>GSHDYLFKLLLIGDSGVGKTCVLFRFSEDAFNSTFISTIGIDFKIRTIELDGKRIKLQIWDTAGQERFRTITTAYYR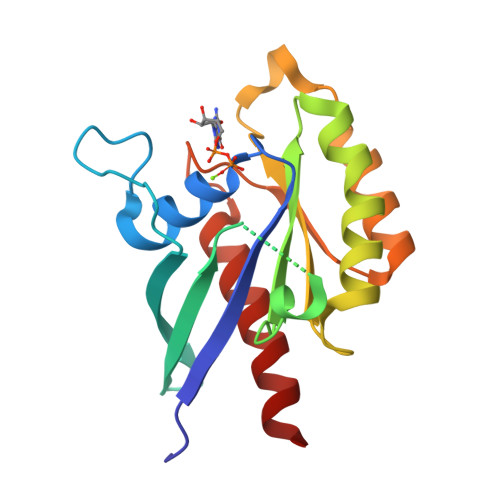GAMGIMLVYDITNEKSFDNIRNWIRNIEEHASADVEKMILGNKCDVNDKRQVSKERGEKLALDYGIKFMETSAKANINVENAFFTLARDIKAKMDKK[5x]methyl ~{N}-[4-aminocarbonyl-1-[(3~{R},4~{R})-4-(cyanomethyl)-1-[(4-ethenyl-2-fluoranyl-5-oxidanyl-phenyl)methyl]-3-fluoranyl-piperidin-4-yl]pyrazol-3-yl]carbamate 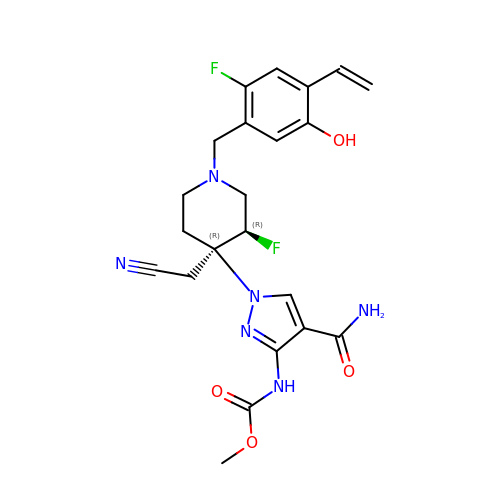| C22 H24 F2 N6 O4 | KNQPQNPPLBJXJR-GCJKJVERSA-N>[2x]MASMTGGQQMGRDPNSLMTNRLVLSGTVCRAPLRKVSPSGIPHCQFVLEHRSVQEEAGFHRQAWCQMPVIVSGHENQAITHSITVGSR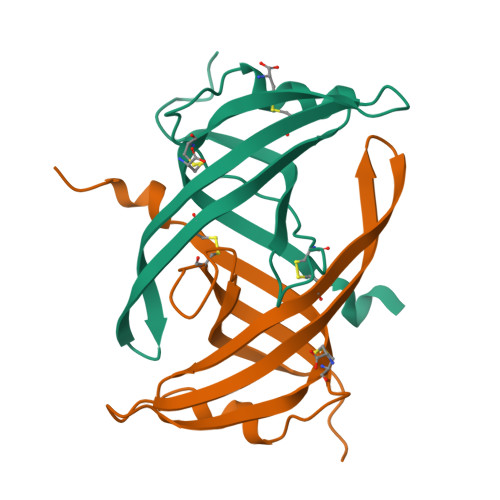ITVQGFISCHKAKNGLSKMVLHAEQIELIDSVDKLAAALEHHHHHH>AGCUU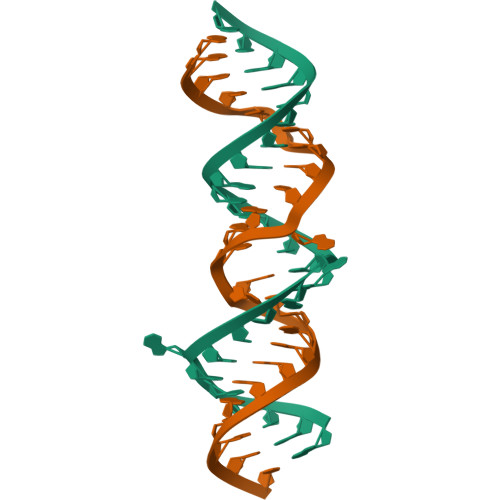GCUUUAAGCCGCUGGAGGAGCU[2x]> MRITIYTRNDCVQCHATKRAMENR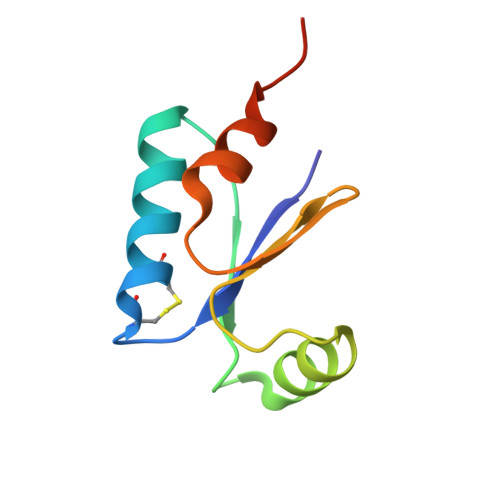GFDFEMINVDRVPEAAEALRAQGFRQLPVVIAGDLSWSGFRPDMINRLHPAPHAASA FORMYCIN B | C10 H12 N4 O5 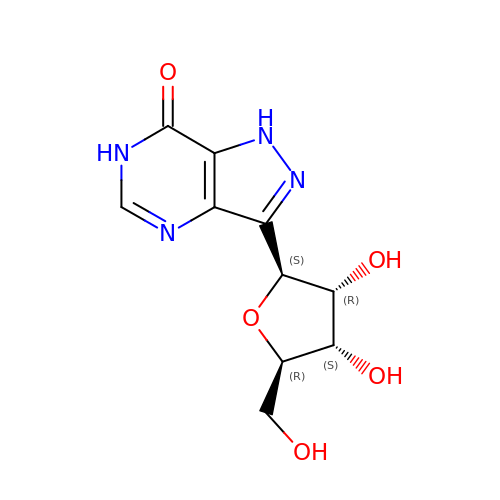| MTCJZZBQNCXKAP-KSYZLYKTSA-N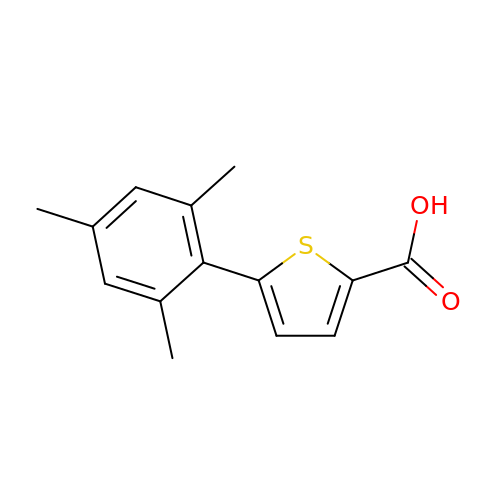5-(2,4,6-trimethylphenyl)thiophene-2-carboxylic acid | C14 H14 O2 S | KRVQNZWUCJAZTJ-UHFFFAOYSA-N>[3x]PSKKNGRSGPQPHKRWVFTLNNPSEDERKKI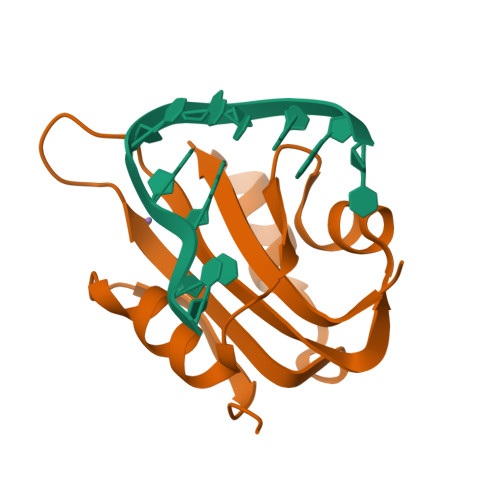RDLPISLFDYFIVGEEGNEEGRTPHLQGFANFVKKQTFNKVKWYLGARCHIEKAKGTDQQNKEFCSKEGNLLMECGAPRSQGQR>[2x]MTQDVTSGYSNLDLDLRDNGVCVVTLNRPDKRNALDVATIEELVTFFSTAHRKGVRAVVLTGAGDHFCAGLDLVEHWKADRSADDFMHVCLRWHEAFNKMEYGGVPIIAALRGAVVGGGLELASAAHLRVMDQSTYFALPEGQRGIFTGGGATIRVSDMIGKYRMIDMILTGRVYQGQEAADLGLAQYITEGSSFDKAMELADKIASNLPLTNFAICSAISHMQNMSGLDAAYAEAFVGGIVNTQPAARERLEAFANKTAARVRPNSLEHHHHHH

The enzyme DmdD catalyzes the last step of the MeSH pathway, the hydration and hydrolysis of MTA-CoA. DmdD belongs to the crotonase superfamily of enzymes, homologous to the equivalent enzyme in the fatty acid β-oxidation pathway. The structure of the DmdD monomer contains two domains. Consistent with the gel-filtration data, DmdD is a hexamer in the crystal, which is also similar to the architecture of canonical crotonases.

The crystal structure of wild-type R. pomeroyi DmdD free enzyme has been determined at 1.5 Å resolution by the molecular replacement method. The hexamer is generated from the two monomers in the asymmetric unit by the crystallographic 3-fold symmetry axis, and can be regarded as two layers of DmdD trimers. The N-terminal domain (NTD) adopts the typical spiral crotonase fold (β-β-αsuperhelix, β1–β11 and α1–α8), which is organized around two roughly perpendicular β-sheets. The C-terminal domain (CTD) consists of three α helices (α9–α11) followed by a long loop at the extreme C-terminus of the protein. The CTD mediates the hexamerization of DmdD, and the long loop at the C-terminus also participates in the formation of the CoA binding site of a neighboring monomer of the hexamer (see below). The active site is located at the trimer interface, and the three active sites in each trimer are identical to each other due to the crystallographic symmetry. There is one striking structural difference, however, between DmdD and ECH. The C-terminal loop (CTL) in ECH is positioned nearly 90° away from that in DmdD. Wild-type DmdD has strong activity toward MTA-CoA, both for MeSH release (equivalent to hydration of MTA-CoA) and for CoA ester hydrolysis. The hydration reaction is analogous to the canonical crotonase enzymes, and likely employs a similar mechanism, with Glu121 as the general base and Glu141 as the general acid.> XPKGRPGPKG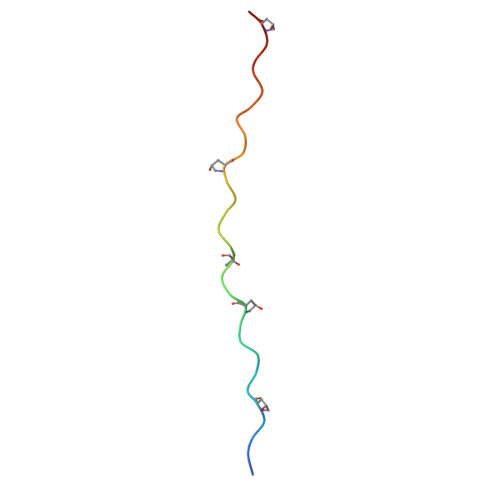FPGYPGPRGRPGKKGPRGPPGX> MFERIDYYAGDPILGLVEKFAADNNPDKVNLGIGIYYDESGVMPVLDCVKIAEQRIADPISPRPYLPMAGLPGHRKGCQELLFGKDAPVLKDGLVATIATIGGSGALKVGAEFIHEWFPQSKCYVSDPTWGNHIAIFEGCDIEVGKYPYYDTATGGIKFDEMIAFFETLNKDDVLLLHPCCHNPTGVDLTREQWDTVLNVIQERELIPFMDIAYQGFGEDMDSDAYAIRKAVDMGLPLFVSNSFSKNLSLYGERVGGLSVVCPTVDETERVFGQLNSTVRRIYSSPPSHGGRVVDIVMNDAALHEQWVGEVYAMRDRIKSMRTKLKSVLEAKISGRNFDYLTAQNGMFSFTGLTPEQVERLQSEFGIYMISNSRMCVAGLNSSNIDYVANAMVDVLKD

The psychrophilic aromatic aminotransferase from Psychrobacter sp. B6 is a representative of pyridoxal phosphate (PLP)-dependent enzymes. PsyArAT exhibits an activity typical for ArAT: transamination, which is a transfer of an amine group between aromatic α-amino acids and α-ketoacids. The mechanism of active site adjustment toward substrates of psychrophilic aromatic amino acid aminotransferase (PsyArAT) from Psychrobacter sp. B6 is discussed based on crystal structures of complexes with four hydroxy-analogs of substrates: phenylalanine, tyrosine, tryptophan and aspartic acid. These competitive inhibitors are bound in the active center of PsyArAT but do not undergo transamination reaction, which makes them an outstanding tool for examination of the enzyme catalytic center.

DL-malic acid sodium salt was used for the PsyArAT/DOH complex creation, but only L-malic acid (DOH) was bound in the active center. The ligand creates considerably more hydrogen bonds than aromatic inhibitors; 10 interactions with residues in the active site were present. Oxygen atoms of the α-carboxylic group of malic acid create strong parallel hydrogen bonds with two nitrogen atoms of the guanidine group from Arg374: (2.8 Å and 2.8 Å). Additionally, they are involved in contact with the amide group of Gly34 (2.8 Å) and Asn183 (3.0 Å). Oxygens of the β-carboxylic group of the ligand interacted, via hydrogen bonds, with Arg280* (2.9 Å and 2.9 Å) and Trp130 (2.8 Å). Hydroxyl oxygen of malic acid creates weak hydrogen bonds with Trp130 (3.2 Å) and stronger bonds with Nζ of Lys246 (2.9 Å). Interaction with Arg280* was of special importance; in this situation, the arginine switch was in the “up” position, and the ligand is shoved further from the entrance; hence, the helix H1 is able to close the active site fully. DOH is a ligand of smaller size than aromatic hydroxy-analogs, and due to interactions with Arg280*, it was shoved deeper in the active site; in this situation, Leu14 moved into the center, enabling proper rotation of H1 and full closure conformation. The small acidic inhibitor (DOH) caused different orientation of the Arg280* and forced closed the conformation of the active center. The functional dimer of the PsyArAT/DOH complex was created from two symmetry-related subunits.> MKLDIKKTFSNRSDRVKGIDFHPTEPWVLTTLYSGRVELWNYETQVEVRSIQVTETPVRAGKFIARKNWIIVGSDDFRIRVFNYNTGEKVVDFEAHPDYIRSIAVHPTKPYVLSGSDDLTVKLWNWENNWALEQTFEGHEHFVMCVAFNPKDPSTFASGCLDRTVKVWSLGQSTPNFTLTTGQERGVNYVDYYPLPDKPYMITASDDLTIKIWDYQTKSCVATLEGHMSNVSFAVFHPTLPIIISGSEDGTLKIWNSSTYKVEKTLNVGLERSWCIATHPTGRKNYIASGFDNGFTVLSLGNDE;> CTFKTKTN

COPI mediates retrograde trafficking from the Golgi to the endoplasmic reticulum (ER) and within the Golgi stack, sorting transmembrane proteins bearing C-terminal KKxx or KxKxx motifs. The heptameric COPI complex (α/β/β'/γ/δ/ε/ζ) is recruited en bloc onto Golgi membranes (Hara-Kuge et al., 1994) but can be divided conceptually into two subcomplexes. The α/β'/ε B-subcomplex has been likened to clathrin because α-COP, β'-COP, and clathrin contain N-terminal WD-repeat (also referred to as β-propeller) domains and C-terminal α-solenoid domains and because recent studies have suggested that β'-COP, like clathrin, can form trimers. We demonstrate that N-terminal WD-repeat domains of α- and β'-COP directly bind dilysine motifs and establish the molecular bases for the interactions using X-ray crystallography, structure-directed mutagenesis, and isothermal titration calorimetry (ITC).

As a result, we used an untagged β'1-304 construct in all further studies and subsequently obtained structures of β'1-304 in complex with CTFKTKTN and CTFKKTN peptides. Because both structures reveal the same mode of binding via the carboxy terminii and -3 lysines of motifs, we present here the structure of β'1-304 with its preferred ligand, CTFKTKTN. All eight residues of the peptide are visible in the 1.8 Å resolution complex. Interaction between β'1-304 and the KxKxx motif is mediated primarily by electrostatic contacts. The peptide carboxy terminus is located on a positively charged patch formed by guanidinium groups of R15 and R59 and the amino group of K17 in the center of the top surface of the WD-repeat domain. The -3 lysine interacts with a negatively charged patch formed from carboxylate groups of D206 and E248. In a negative patch formed by D98 and D117, a lysine residue (K261) from a symmetry copy of the domain has displaced the -5 lysine found in the peptide motif. The second critical crystal contact is a disulfide bond formed by oxidation between the peptide cysteine and C220 in a symmetry copy of β'1-304. The final key structural feature is the location of the -2, -3, and -4 carbonyl groups of the motif, which project down into a basic groove. The structure of KxKxx motifs bound to the N-terminal WD-repeat domain of β'-COP identifies electrostatic contacts between the motif and complementary patches at the center of the β'-COP propeller.N-[(2R,3S)-1-((2S)-2-{[(CYCLOPENTYLAMINO)CARBONYL]AMINO}-3-METHYLBUTANOYL)-2-(1-FORMYL-1-CYCLOBUTYL)PYRROLIDINYL]CYCLOPROPANECARBOXAMIDE | C24 H38 N4 O4 | 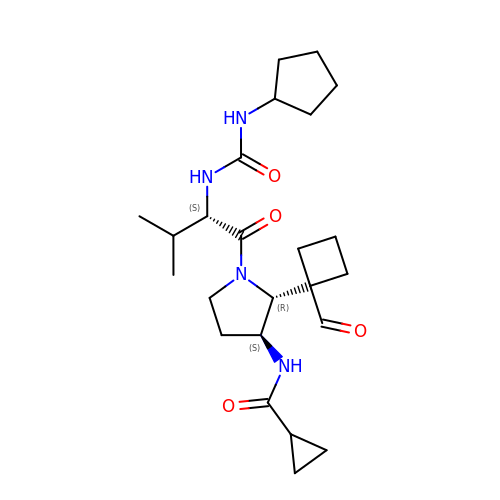GCDRFILPPBOJLM-UFYCRDLUSA-N Vertebrates have two highly related Rock proteins, Rock1 and Rock2, which share 65% sequence identity to each other. Both contain an N-terminal kinase domain, a centrally located coiled coil region and C-terminal pleckstrin homology (PH) and cysteine-rich domains. Rock catalytic activity is inhibited by a direct intramolecular interaction between the kinase domain and sequences within a large C-terminal fragment of Rock containing 200 residues of the coiled-coil region, the PH domain , and the cysteine-rich domain. To accomplish this task, Shrm3 is localized to apically positioned sites of cell-cell adhesion in polarized cells, where it directly interacts with Rock through a highly conserved domain on its C-terminus called the Shrm Domain 2 (SD2).

While binding affinity was somewhat reduced in this assay for the smaller 834–913 fragment, both Rock1 proteins were still capable of binding SD2 with affinities comparable to that observed between Drosophila Rock and Shrm. Together, these data suggest that there is a stable Shrm binding domain (SBD) composed of residues 834–913 of hRock1. Diffraction quality was greatly improved through the introduction of a triple alanine mutation, 884EKE886, suggested by the Surface Entropy Reduction server and termed SBDSER. Crystals of SBDSER belong to space group C21 and also exhibit anisotropy with diffraction extending to 2.5 Å along a* and c* but only 3.1 Å along the b* plane. Phases were determined using the SAD method, and the final model was refined against native data at 2.5 Å resolution to Rwork and Rfree values of 23.6% and 27.6% respectively. SBDSER crystals contain two parallel coiled-coil dimers in the asymmetric unit packed in a tail-to-tail arrangement. Each SBD monomer is an entirely helical segment ∼100 Å in length and the completed model minimally contains residues 838–902 from each molecule. The C-terminal end of each dimer is splayed open allowing the formation of a helical bundle beginning at residue 875. The SBDSER mutant that facilitates crystallization, positions 884–886, is located within the center of this helical bundle. The helix is noticeably kinked after the SBDSER positions suggesting that the substitutions at the SBDSER positions may have altered the overall structure of the SBD to favor the formation of a helical bundle between residues 875–902. Since SBDSER is dimeric in solution, crystal packing forces, perhaps accentuated by additional hydrophobic interactions found in the SBDSER variant, are likely responsible for the observed helical bundle.

>[4x]GIDPFTGNEGQMRELQDQLEAEQYFSTLYKTQVKELKEEIEEKNRENLKKIQELQNAAATLATQLDLAETKAESEQLARGLLEEQYF> MGHHHHHHHHHHSSGHIDDDDKMKVLTELQKQIFTIVKK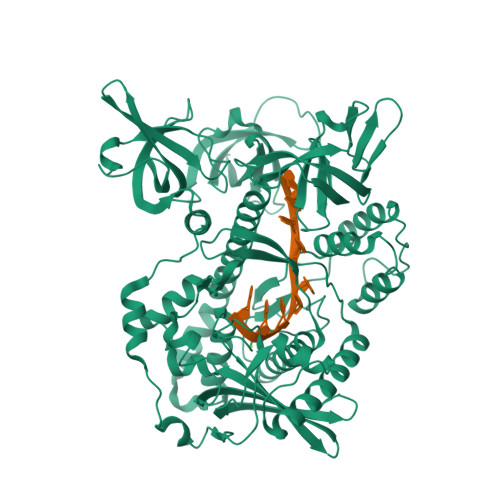ENGKPIPPGIVVRMMENSPNFPGKHLIYRAIDDLLDWAILRKAGGVTNQLLVNYEPAEPLLDKKLQGILTLGNKNSGFIRSLDDDKTVYYVHYSNLTGALDGDLVEFCKLDKPQFGDKFDAAVITILKRARILYAGNFLVDQNEFALEYKIVADNPRFYLTMIVNPDSIPNNLASNTKIAFQIDEYDPDNNLCKVSVQQVLGNNDDPLINIKAIMLDNSIVFETNDVVEQHANKLSFDTEEQHKAYRQDLTDLAFVTVDPTTSKDLADAIYVKTIPTGFVLYVAIADVAHYVNRNSEIDIEAKHKTSSIYLPGHYVVPMLPEQLSNQLCSLNPAQKRYVVVCEISFDNQGRIKTNKLYPATIISKNRFSYDQVNKWLNNKSELNCDETVINSLKAAFTLSDLIQAQRQKRGTIDLSHKETEIVVDEHYFPIKINFLVHDKAETMIENLMVVANETVAWVLTNNKIALPYRVHPRPSKKKLQSLIETVGELNITKPQFNLDTVTSSQIASWLNENKDNPSYEIFVILLLRTLGKAFYSVNPLMHFSIGSNHYTHFTSPIRRYIDLTIHRLLWMHLFTPDQFTDNERDQLKQELEKIADTVNDTEIKIINCERNANDYLTTLLLSKQIGKTFSGFISAITSFGIFMRMDENNFDGLIKITTIPDDFFIFEKEKMVLKGRKTNKVYKIGDRLEAKLSEIDFIQKRAILTLI> MRCLALDIGGTKIAAAIVKNGEIEQRQQIHTPRENVVEGMHQALGKLLADY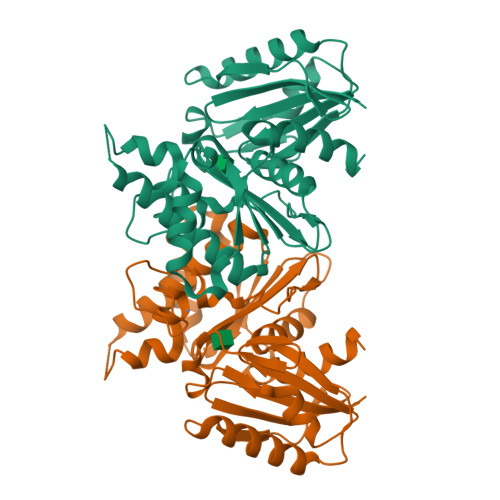EGQFDYVAVASTGIINNGILSALNPKNLGGLAEFPLKASIAKHTDKPIGLLNDAQAATYAEYQLQNFEQVSNFVFITVSTGVGGGIVLNQILQTGSRGIAGHIGHTLADPNGAICGCGRRGCVEAIASGRAIEAVSSQWEDPCDPKEVFERFRKNDEKATALVERSAKAIANLIADLVISLDIQKIAIGGSVGLAEGYLSLVEKYLQDFPSIYCCEIETAKFGQDAGLIGAAYWVKDVL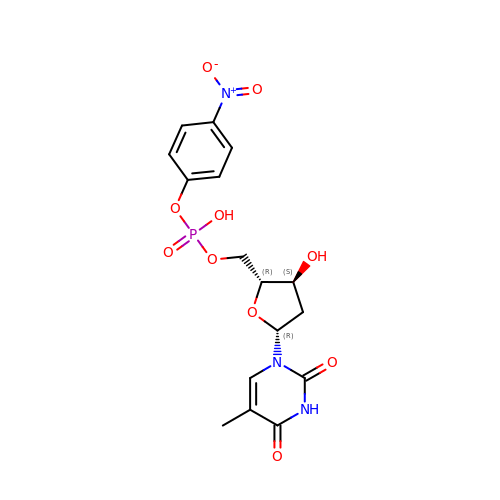5'-O-[(S)-hydroxy(4-nitrophenoxy)phosphoryl]thymidine | C16 H18 N3 O10 P | RWOAVOYBVRQNIZ-BFHYXJOUSA-N>MKLPIYLDYSATTPVDPRVAEKMMQFMTMDGTFGNPASRSHRFGWQAEEAVDIARNQIADLVGADPREIVFTSGATESDNLAIKGAANFYQKKGKHIITSKTEHKAVLDTCRQLEREGFEVTYLAPQRNGIIDLKELEAAMRDDTILVSIMHVNNEIGVVQDIAAIGEMCRARGIIYHVDATQSVGKLPIDLSQLKVDLMSFSGHKIYGPKGIGALYVRRKPRVRIEAQMHGGGHE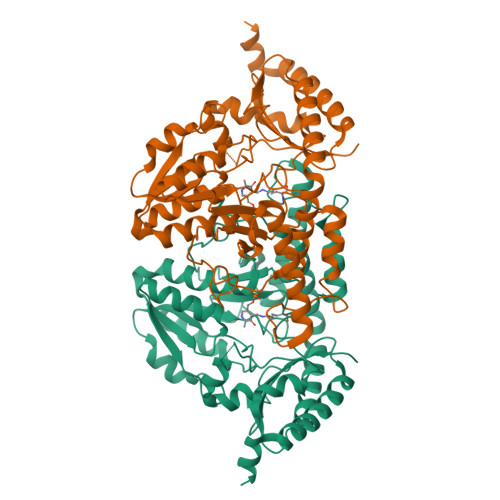RGMRSGTLPVHQIVGMGEAYRIAKEEMATEMERLRGLRNRLWNGIKDIEEVYLNGDLEHGAPNILNVSFNYVEGESLIMALKDLAVSSGSACTSASLEPSYVLRALGLNDELAHSSIRFSLGRFTTEEEIDYTIELVRKSIGRLRDLSPLWEMYKQGVDLNSIEWAHH[2x]> GSPALDTGTTEEDRLKIDVIDWLVFDPAQRAEALKQGNAIMRKFLASKKHEAAKEVFVKIPQDSIAEIYNQCEEQGMESPLPAEDDNAIREHLCIRAYLEAHETFNEWFKHMNSVPQKPALIPQPTFTEKVAHEHKEKKYEMDFGIWKGHLDALTADVKEKMYNVL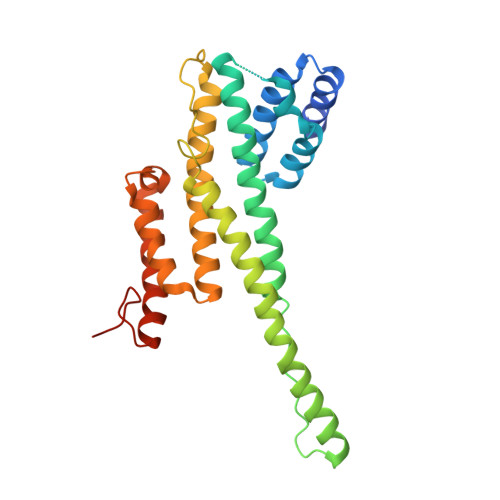LFVDGGWMVDVREDAKEDHERTHQMVLLRKLCLPMLCFLLHTILHSTGQYQECLQLADMVSSERHKLYLVFSKEELRKLLQKLRESSLMLLDQGLDPLGYEIQLSGRIVTD>GARRFLCGVVEGFYGRPWVMEQRKELFRRLQKWELNTYLYAPKDDYKHRMFWREMYSVEEAEQLMTLISAAREYEIEFIYAISPGLDITFSNPKEVSTLKRKLDQVSQFGCRSFALLFDDIDHNMCAADKEVFSSFAHAQVSITNEIYQYLGEPETFLFCPTEYCGTFCYPNVSQSPYLRTVGEKLLPGIEVLWTGPKVVSKEIPVESIEEVSKIIKRAPVIWDNIHANDYDQKRLFLGPYKGRSTELIPRLKGVLTNPNCEFEANYVAIHTLATWYKSNMNGVRKDVVMTDSEDSTVSIQIKLENEGSDEDIETDVLYSPQMALKLALTEWLQEFGVPHQYSSR[2x];>[2x]MEKPLYTAEPVTLEDLQLLADLFYLPYEHGPKGAQMLREFQWLRANSSVVSVNCKGKDSEKIEEWRSRAAKFEEMCGLVMGMFTRLSNCANRTILY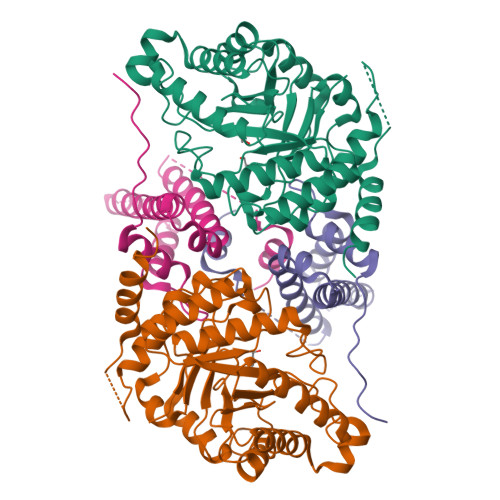DMYSYVWDIKSIMSMVKSFVQWLGCRSHSSAQFLIGDQEPWAFRGGLAGEFQRLLPIDGANDLFFQP>MAIAHIATEYVFSDFLLKDPPESKYKGLRLELAVDKLVSCIAVGLPLLLISLAFAQEITLGSQISCFAPTSFSWRQAAYVDSFCWAAVQQKHLSQSDSGNVPLWLHKFFPYILLLVAVLLYLPNLFWRFTAAPHLSSDLKFVMEELDKCYNRDIKDIKAANNLNSSDKRDGLNSPVVSENLQQSLWEIPLSHYKYPIVEQYLKTKNNSYGLIIKYLICRVVTLIIVFTACIYLGYYISLFSLTDEFTCNIRTGILRNDTALPPLVQCKLIAVGVFRLLSYINLIIYVLIMPFIIYAMLVPFRKTANVLKVYEVLPTFSVQQAPSKTYDDHSLFLLFLEENVSELKSYKFLKVLENIKNTGENFDTIQYLTSLGTVKTDTVDGKLAFKCTSEVPNNTEQNEVELTVQPSSDNAKTEEKKVRQRLLDSSCSNS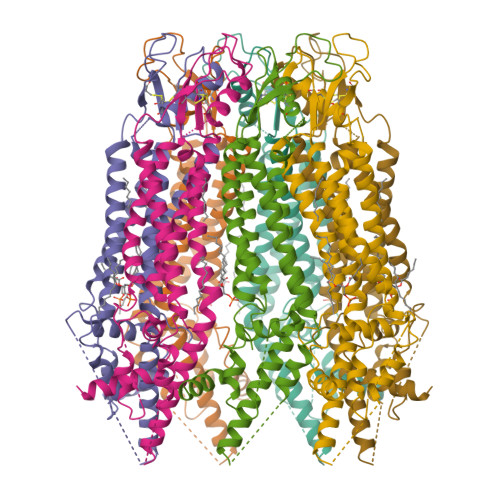LEVLFQ[7x]(1S,2S,3R,6R)-6-[(2-hydroxybenzyl)amino]cyclohex-4-ene-1,2,3-triol 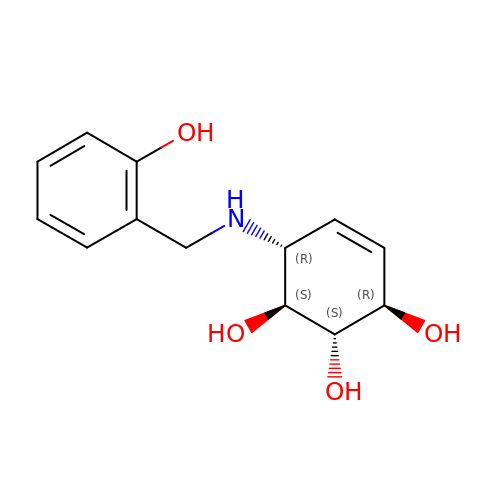| C13 H17 N O4 | IXUCFEUMPUFAGK-XEZLXBQYSA-N N-[(1S,2S)-1-[(3R,6R)-6-(cyclohexylmethoxy)morpholin-3-yl]-3-(3,5-difluorophenyl)-1-hydroxypropan-2-yl]acetamide | C22 H32 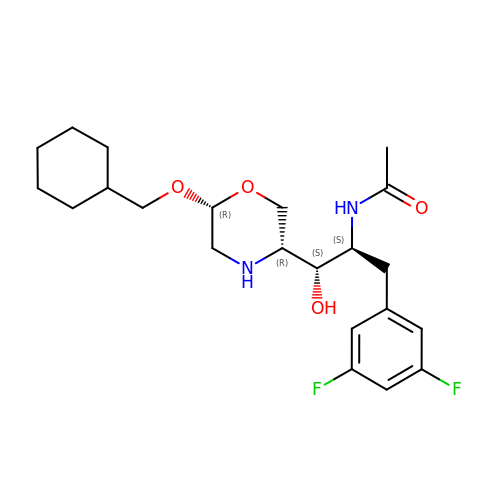F2 N2 O4 | XQHQHHREHKYCIG-CBPXPLCBSA-N>MSAKPQPIAAAAWKCN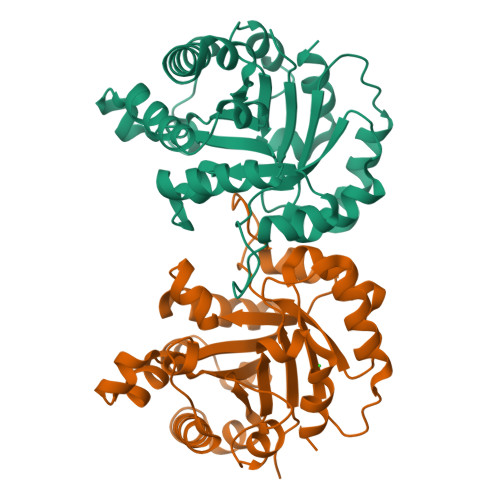GTTASIEKLVQVFNEHTISHDVQCVVAPTFVHIPLVQAKLRNPKYVISAQNAIAKSGAFTGEVSMPILKDIGVHWVILGHSERRTYYGETDEIVAQKVSEACKQGFMVIACIGETLQQREANQTAKVVLSQTSAIAAKLTKDAWNQVVLAYEPVWAIGTGKVATPEQAQEVHLLLRKWVSENIGTDVAAKLRILYGGSVNAANAATLYAKPDINGFLVGGASLKPEFRDIIDATR[4x]β-prism folds in V. cholerae are not unique to VCC: three additional β-prism domains exist in two biofilm matrix proteins called RbmC (rugosity and biofilm structure modulator C) and Bap1 (biofilm associated protein 1). RbmC and Bap1 are related multidomain proteins with overlapping functions, involved in the surface attachment of biofilms and encapsulation of growing cell clusters. For simplicity, we refer to the two β-prism domains of RbmC as RbmC1 and RbmC2. Our results illustrate a common structural mechanism by which vibrio toxin and biofilm β-prism domains target glycans on host cell-surfaces, facilitating cell lysis in one case and cell attachment in another.

RbmC2 apo crystals were obtained with space group C2221, with three copies in the asymmetric unit. In the apo structure (with three protein molecules in the asymmetric unit), glycerol molecules from the cryo-protection solution are found in the glycan binding pocket. In two copies of the asymmetric unit, a water is present bound to W948 as in the mannotriose and GlcNAc-Man structures. In the third copy, a hydroxide group from a glycerol molecule replaces this position. As previously stated, the loop containing the N871 residue is unstructured in two of three copies of the asymmetric unit and the ordered copy is in a different conformation than in the ligand-occupied structures. This suggests that binding of the ligand may lead to the ordering of this loop and that the water molecule coordinated by N871 and W948 may help mediate this interaction. Comparing glycan-bound structures to the three copies of RbmC2 in the apo structure asymmetric unit revealed differences in a loop (with the sequence PVQGT), which is not present in the other vibrio lectin domains. Aside from the rearrangement of this loop, only subtle side-chain rearrangements of F850, W896, and W948 are observed between the apo and mannotriose-bound, and GlcNAc-Man-bound structures. The all-atom RMSD between the two ligand-bound structures is 0.21 Å2 and approximately 0.34 Å2 between liganded and apo (compared to 1.2 Å2 for RbmC2 vs. VCC β-prism).

>[3x]AMGSPIFGYSNTQQSQRVVTADNLMYLRSGFAIDAIGTTVNNLVGGPVQGTNGGVLRAPIALDQLQSVEVTSGLYNWGGYHIVAIKFTMKDGSSVLLGSTHYASNKKVETYTVPQGKRIKQINVWTGGWLVEGFQFVY>MRIQVNAKGAARLLSRHLWVFRRDVVSGPETPGLYPVYWGRRFLALALYNPHTDLAVRAYRFAPAEDPVAALLENLAQALARREAVLRQDPEGGYRLVHAEGDLLPGLVVDYYAGHAVVQATAHAWEGLLPQVAEALRPHVQ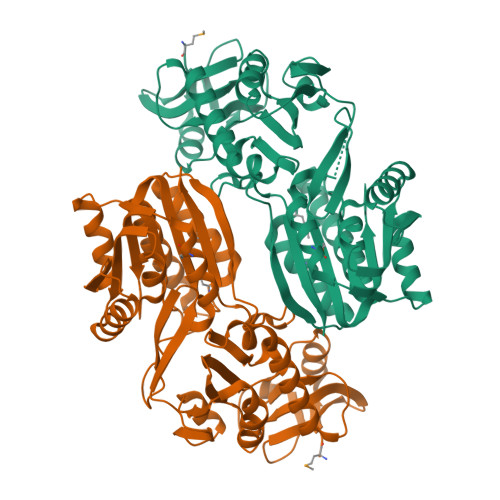SVLAKNDARTRELEGLPLYVRPLLGEVPERVQVQEGRVRYLVDLRAGQKTGAYLDQRENRLYMERFRGERALDVFSYAGGFALHLALGFREVVAVDSSAEALRRAEENARLNGLGNVRVLEANAFDLLRRLEKEGERFDLVVLDPPAFAKGKKDVERAYRAYKEVNLRAIKLLKEGGILATASCSHHMTEPLFYAMVAEAAQDAHRLLRVVEKRGQPFDHPVLLNHPETHYLKFAVFQVL[4x]3-(4-aminophenyl)benzoic acid 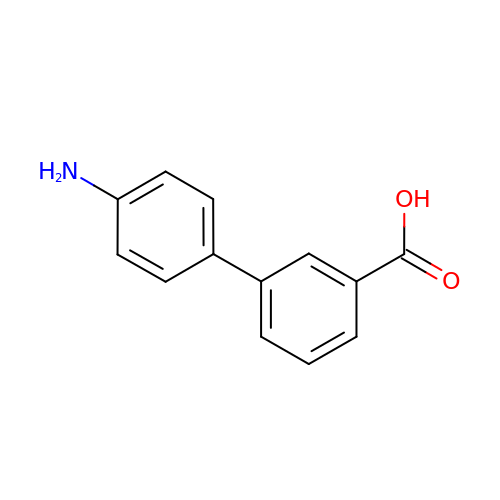| C13 H11 N O2 | AZMVFOPKHNNXDO-UHFFFAOYSA-N>[2x]MGSSHHHHHHSSGRENLYFQGHERLTLDTRLRQALERNELVLHYQPIVELASGRIVGGEALVRWEDPERGLVMPSAFIPAAEDTGLIVALSDWVLEACCTQLRAWQQQGRAADDLTLSVNISTRQFEGEHLTRAVDRALARSGLRPDCLELEITENVMLVMTDEVRTCLDALRARGVRLALDDFGTGYSSLSYLSQLPFHGLKIDQSFVRKIPAHPS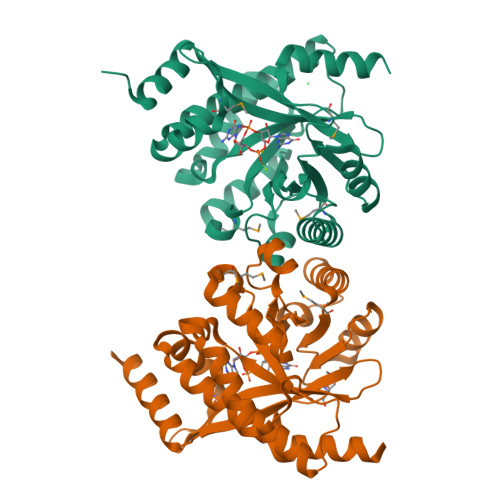ETQIVTTILALARGLGMEVVAEGIETAQQYAFLRDRGCEFGQGNLMSTPQAADAFASLLDRQKASGQRPVHGHETAP>MGAMIVKEVYETAEKIKSMEIRGAGRIARAAAQALMIQAEKSKAKEPEELWNELKVASKILYNTRPTAVSLPNALRYVMHRVKAAYLGGADLETLRFTAINSAKEFIYNSEKAIERIGEIGAKRIEDGDIIMTHCHSKAAISVMKKAFEQGKNIKVIVTETRPKWQGKITAKELASYGIPVIYIVDSAARHYMKMTDKVVMGADSITANGAVINKIGTSLIALTAKEHRVWVMIAAETYKFHPATMLGQLVEIEMRDPTEVIPEEELRTWPKNIEVWNPAFDVTPPEYIDVIITERGIIPPYAAIDILKEEFGWALKYKEPWED[3x]

In summary, our study demonstrates that PH0208 protein would function as a purine nucleotide dependent R15Pi enzyme and not as a homologue of the regulatory subunit of eIF2B. In NMP degradation pathway, R15Pi catalyzes the conversion of ribose-1,5-bisphosphate (R15P, substrate) into ribulose-1,5-bisphosphate (RuBP, product) in an adenosine 5′-monophosphate (AMP)-dependent manner. AMP acts as an activator of R15Pi and in its absence the enzymatic activity has been found to decline dramatically. Monomer of PH0208 protein consists of an N-terminal α-helical domain (residues 1–122) and a C-terminal α-β-α sandwich domain (residues 123–324).

One asymmetric unit (ASU) consists of three identical (root mean square deviation, RMSD: 0.16 Å for 321 Cα atoms of 324 residues) subunits of the protein. The active site pocket of PH0208 protein resides in the cavity formed between the N- and C-terminal domains and was found to hold the product (RuBP) indicating that the substrate was converted into product during the process of crystallization. However, unlike the homologous proteins, PH0208 remains in a closed conformation even when the product is bound to the active site. This closed conformation is reflected by the bend angle of the α5 helix, which is ~10° for the closed conformation. In the active site pocket, the 1-phosphate group of RuBP forms hydrogen bond to the side chains of the residues Arg22, Arg65, Gln166, Lys215 and the backbone amide group of Gly23. The 5-phosphate group forms hydrogen bond to the side chains of the residues Ser137, Lys240 and the backbone amide group of Ala24, Gly25, Lys138 and Ala139. The side chain atoms of Asp204, Asn214 and Lys215 interact with the oxygen atoms of the ribulose sugar. The amino acid residues of PH0208 protein involved in interacting with the 1-phosphate, sugar and 5-phosphate group of RuBP are well conserved in all R15Pi enzymes. However, the strong binding of the substrate/product of R15Pi enzyme to the active site pocket of PH0208 protein by forming interactions with all the crucial and conserved amino acid residues clearly indicates that PH0208 protein would function as R15Pi.The earlier discovery of the pathway responsible for alkane biosynthesis in cyanobacteria allowed the conversion from solar energy to alkanes through photosynthesis, without providing external carbon sources. This two-step pathway utilizes two water-soluble enzymes, namely acyl-acyl carrier protein (acyl-ACP) reductase (AAR) and aldehyde-deformylating oxygenase (ADO). AAR catalyzes the first step of this pathway, reducing the substrate fatty acyl-ACP/fatty acyl-coenzyme A (acyl-CoA) into the corresponding aldehyde in a NADPH-dependent manner. Subsequently, ADO catalyzes the conversion of fatty aldehyde into alk(a/e)ne with one carbon shorter (Cn-1 hydrocarbon) and the formate as a C1-derived form. Here we report the crystal structure of AAR from Synechococcus elongatus PCC 7942 (SeAAR) in its apo form (AARapo), together with three structures of AAR in complex with ADO from the same species of cyanobacteria (SeADO), in which AAR binds either substrate or substrate/cofactor.

In order to identify the NADPH binding pattern, we either co-crystallized AAR or soaked the AAR–ADO crystals with NADPH, and finally solved the AARNADPH–ADO structure at 2.1 Å resolution by soaking the AARthioester–ADO crystal with NADPH. In the structure, one NADP(H) molecule is accommodated in the hydrophilic cleft above C294, and is mainly stabilized by the mid-domain of AAR. The ADP moiety is sandwiched by the dinucleotide recognition loop and the 222VASM225 loop region within Fr-III. The 3′-phosphate group of the ADP moiety is located in a pocket surrounded by three positively charged residues: R189, R193, and R314. In the AARNADPH–ADO structure, the nicotinamide moiety of NADPH is located close to C294 of AAR, with its C4 atom being located only 3.14 Å away from the stearoyl-C1 atom. The short distance supports the possibility that C4 of NADPH provides a hydride to break the thioester bond. The stearic chain is located in the acyl-tunnel of AAR, as was observed in the AARthioester–ADO structure. However, the weaker electron density of the stearic chain in the AARNADPH–ADO structure suggests that it only partially occupies the acyl-tunnel. Subsequently, NADPH is incorporated into the cleft above C294 of AAR (S3, represented by the AARNADPH–ADO structure), before AAR catalyzes the hydride transfer of NADPH, and before reduction of the acyl moiety to a long-chain aldehyde.

> MFGLIGHLTSLEQARDVSRRMGYDEYADQGLEFWSSAPPQIVDEITVTSATGKVIHGRYIESCFLPEMLAARRFKTATRKVLNAMSHAQKHGIDISALGGFTSIIFENFDLASLRQVRDTTLEFERFTTGNTHTAYVICRQVEAAAKTLGIDITQATVAVVGATGDIGSAVCRWLDLKLGVGDLILTARNQERLDNLQAELGRGKILPLEAALPEADFIVWVASMPQGVVIDPATLKQPCVLIDGGYPKNLGSKVQGEGIYVLNGGVVEHCFDIDWQIMSAAEMARPERQMFACFAEAMLLEFEGWHTNFSWGRNQITIEKMEAIGEASVRHGFQPLALAIENLYFQ;> MRTPWDPPNPTFSLSSVSGDRRLMPQLEASLELDFQSESYKDAYSRINAIVIEGEQEAFDNYNRLAEMLPDQRDELHKLAKMEQRHMKGFMACGKNLSVTPDMGFAQKFFERLHENFKAAAAEGKVVTCLLIQSLIIECFAIAAYNIYIPVADAFARKITEGVVRDEYLHRNFGEEWLKANFDASKAELEEANRQNLPLVWLMLNEVADDARELGMERESLVEDFMIAYGEALENIGFTTREIMRMSAYGLAAV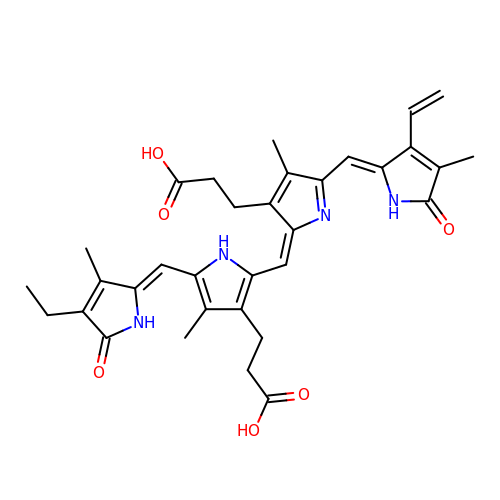3-[2-[(Z)-[3-(2-carboxyethyl)-5-[(Z)-(3-ethenyl-4-methyl-5-oxo-pyrrol-2-ylidene)methyl]-4-methyl-pyrrol-2-ylidene]methyl]-5-[(Z)-(4-ethyl-3-methyl-5-oxo-pyrrol-2-ylidene)methyl]-4-methyl-1H-pyrrol-3-yl]propanoic acid | C33 H36 N4 O6 | PSKIZABPQHQTFV-SRVCBVSDSA-N> GSHMTTTEAGASAPSPAVDGAVNQTARQAEADGTDIVTDHDRGVHGYHKQKAEHLKRLRRIEGQIRGLQRMVDEDVYCIDILTQVSASTKALQSFALQLLEEHLRHCVADAALKG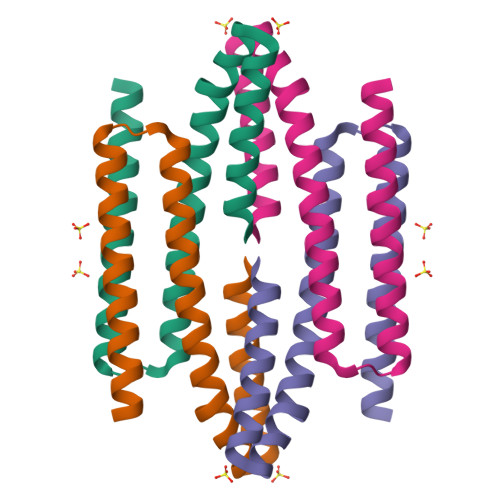GTEIDAKVEEATKAIGRLLRT[2-CYTIDYLATE-O'-PHOSPHONYLOXYL]-ETHYL-TRIMETHYL-AMMONIUM | C14 H26 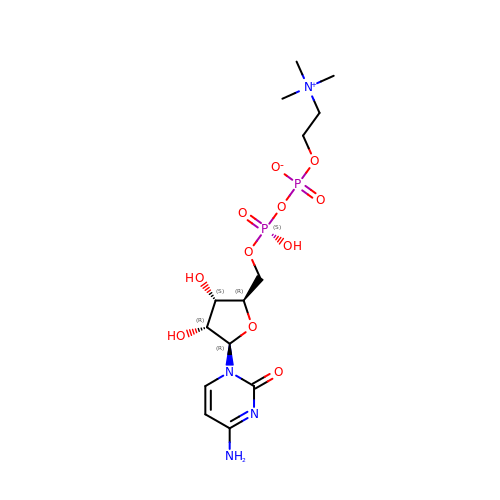N4 O11 P2 | RZZPDXZPRHQOCG-OJAKKHQRSA-N Here we characterize a novel cystatin-type protease inhibitor, mialostatin, from the I. ricinus midgut. Cystatins are tight binding, reversible inhibitors of legumain and papain-like cysteine proteases. Recombinant mialostatin inhibited a number of I. ricinus digestive cysteine cathepsins, with the greatest potency observed against cathepsin L isoforms, with which it co-localized in midgut digestive cells. Mialostatin localized to both digestive cells and the gut lumen, where it targets cathepsin L isoforms and regulates their activity during trafficking and processing of host blood proteins.

The crystal structure of mialostatin was determined by molecular replacement using the structure of the tick cystatin OmC2 as a search model and refined using data to 1.55 Å resolution. The hexagonal prism crystal form contained two molecules in the asymmetric unit with a solvent content of about 57%. All protein residues could be modeled into a well-defined electron density map with the exception of the first nine residues, which formed a flexible N-terminus (Ser1 to Gly9), and the last two C-terminal residues (Asn118, Val119) of chain A. The final model consisted of two mialostatin molecules, chains A and B, containing 108 and 110 residues, respectively. The molecule adopts a typical cystatin fold (so called ‘hot dog’ fold) characterized by a five-stranded twisted antiparallel β-sheet wrapped around a central α-helix. Mialostatin contains two conserved disulfide bridges connecting Cys69 with Cys82 and Cys93 with Cys113. The closest structural homolog of mialostatin was the salivary/gut cystatin OmC2 from the soft tick O. moubata with the highest sequence identity (53%) and lowest RMSD for Cα (0.86 Å), followed by salivary homologs iristatin (41% identity, 1.56 Å RMSD) from the hard tick I. ricinus and sialostatins L1 (42%, 2.09 Å) and L2 (40%, 2.50 Å) from the hard tick I. scapularis. The interaction between family 2 cystatins and papain-type cysteine proteases is mediated by three regions, the N-terminal segment and two hairpin loops L1 and L2, which form a tripartite wedge-shaped edge that binds to the enzyme active site cleft. In mialostatin, the first part of the binding site is formed by the N-terminal segment around Gly10, which is the first visible residue in the electron density map. The L1 loop (between β1 and β2) of mialostatin exposes the segment Gln51-Ile52-Val53-Ala54-Gly55 corresponding to the critical binding motif Gln-Xaa-Val-Xaa-Gly conserved in cystatins. The L2 loop (between β3 and β4) is characterized in mialostatin and other cystatins, except sialostatins, by the presence of a conservative Pro101-Trp102 segment.

>[2x]MDICWNSPLFLVCVVLAAAGSASRSKRALVGGWKTQDPTNPKFENLAHYAVSTQVEGREYYDTVLELLEVQTQIVAGVNYKLKFTTTQSTCKIESGVEYSKELCQPKTNKVEAVCTSIIYTVPWQNIKRVLSYHCDAPNNV Enzymes of the vanillyl alcohol oxidase/p-cresol methyl hydroxylase (VAO/PCMH) superfamily are found across all kingdoms where they perform a range of metabolic functions. These flavoproteins share a conserved FAD-binding domain and a more variable substrate-binding domain that enables interactions with a range of substrates. One of these, the 4-phenol oxidases/dehydrogenases, catalyzes the oxidation of para-substituted phenolic compounds. A fundamental distinction is that the oxidases efficiently react with oxygen producing hydrogen peroxide whereas the dehydrogenases hardly react with oxygen and typically employ other proteins, such as cytochrome c, as acceptors.

Among the proteins of this unexplored clade, we chose the enzyme from Marinicaulis flavus for experimental evaluation. The absorbance spectrum suggests that vanillin (peak at 340 nm) is produced, though the presence of the quinone methide intermediate (peak at 360 nm) remaining bound to a fraction of the protein molecules cannot be ruled out. These features are consistent with molecular oxygen being an inefficient oxidant for the enzyme that is therefore identified as a vanillyl-alcohol dehydrogenase active on the typical substrates of the 4-phenol oxidizing subgroup. To pinpoint structural differences induced by Pro151 mutations, we crystallized VAD and solved its structure. With 46% sequence identity and a root mean square deviation of 0.89 Å for the Cα atoms, its structure closely resembles that of VAO. Conserved features include the dimeric arrangement, a large chamber at the subunit interface, a constellation of active site Arg and Tyr residues, and the substrate binding mode in front of the flavin si side. Pro151 is located within a sharp loop that covers the flavin edge on the re side of the cofactor ring. The residue is in the cis conformation with its carbonyl oxygen atom pointing towards the flavin N5 atom. Conversely, no tunnels are present in the wild type and the dehydrogenase mutants where the flavin re face remains fully shielded by residue 151 and Trp153. We found that wild-type VAD is anaerobically reduced by vanillyl alcohol with a reduction rate constant (kred) of 0.50 s-1 (reductive half-reaction). Specifically, the re-oxidation of the dithionite-reduced enzyme is 52-fold faster than that of the substrate-reduced protein (kox of 14000 vs 27 M-1 s-1).

>[3x]MAAPLPEGVSAEAMSSALDRFARIVGADWVFTEDKITPYEDPYTISNDETEHRPYAAVAPASTEEVQEIVRVANEFGVPLWPVSRGKNFAYGGAAPVMSGTVVLDMNRMNRILEVNEEFGYALVEPGVSYFELYDYIQEKGLKLWIDVPDPGWGSVVGNALDHGIGYTPYGDHFAMQCGMEVVLPNGEVVRTGMGAMPGNNTWQLFKYGYGPYVDGIFSQSNFGVVTKMGIWLMPEPAGYRPYLITFENEDDIETVTERLRPLKVAGVIQNGATVRSLVLDAAITRTKSQYYDGDGPIPPSVAKTMMADLDLGMWNFCGALYGPPPVMDTLWTAIRDSFADIPGVKFYFPEDRRHKVDLLLHRAETMKGVPKLTEFNFLNWDGGGGHVGFSPVSPITGKDAIKQYNMVSSRVREYGFDYMGLLAIGWRDLHHVTVIVYDKTDPDERKKLDELFNILVDEAAAEGYGEYRTHIRYMDRIAKTYSWNDNALWKMHETIKDALDPNGILAPGKSGIWGKNRRKA>MPPYTVVYFPVRGRCAALRMLLADQGQSWKEEVVTVETWQEGSLKASCLYGQLPKFQDGDLTLYQSNTILRHLGRTLGLYGKDQQEAALVDMVNDGVEDLRCKYVSLIYTNYEAGKDDYVKALPGQLKPFETLLSQNQGGKTFIVGDQISFADYNLLDLLLIHEVLAPGCLDAFPLLSAYV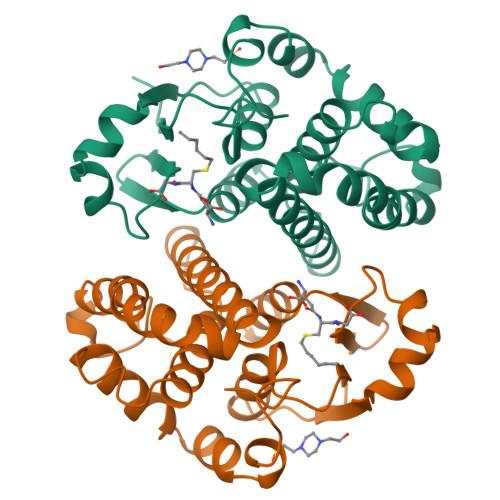GRLSARPKLKAFLASPEYVNLPINGNGKQ[2x]>[2x]GAMGSESLSPGGPPGHPYQGEASTCWQLTVRVLEARNLRWADLLSEADPYVILQLSTAPGMKFKTKTLTDTSHPVWNEAFRFLIQSQVKNVLELSIYDEDSVTEDDICFKVLYDISEVLPGKLLRKTFSQSPQGEEELDVEFLMEETSDRPENLITNKVIVARELSCLDVHLDSTGSTAVVADQDKLELELVLKGSYEDTQTSFLGTASAFRFHYMAALETELSGRLRSSRSNGWNGDNSAGYLTVPLRPLTIGKEVTMDVPAPNAPGVRLQLKAEGCPEELAVHLGFNLCAEEQAFLSRRKQVVAKALKQALQLDRDLQEDEVPVVGIMATGGGARAMTSLYGHLLALQKLGLLDCVTYFSGISGSTWTMAHLYGDPEWSQRDLEGPIRYAREHLAKSKLEVFSPERLASYRRELELRAEQGHPTTFVDLWALVLESMLH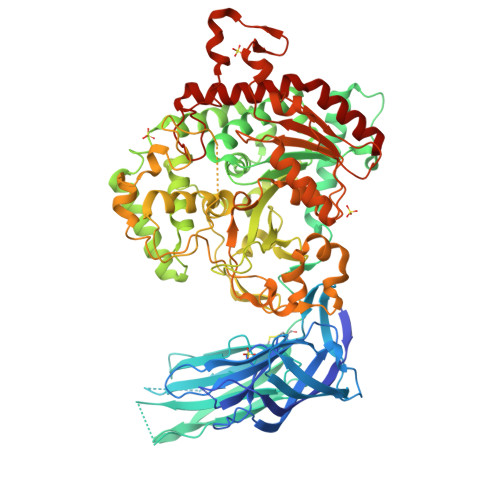GQVMDQKLSGQRAALERGQNPLPLYLSLNVKENNLETLDFKEWVEFSPYEVGFLKYGAFVPPELFGSEFFMGRLMRRIPEPRICFLEAIWSNIFSLNLLDAWYDLTSSGESWKQHIAAATRSLEKEPLTTSGTSSRLEASWLQPGTALAQAFKGFLTGRPLHQRSPNFLQGLQLHQDYCSHKDFSTWADYQLDSMPSQLTPKEPRLCLVDAAYFINTSSPSMFRPGRRLDLILSFDYSLSAPFEALQQTELYCRARGLPFPRVEPSPQDQHQPRECHLFSDPACPEAPILLHFPLVNASFKDHSAPGVQRSPAELQGGQVDLTGATCPYTLSNMTYKEEDFERLLRLSDYNVQTSQGAILQALRTALKHRTLE(S)-2-((3-(6-amino-9H-purin-9-yl)propyl)amino)-3-phosphonopropanoic 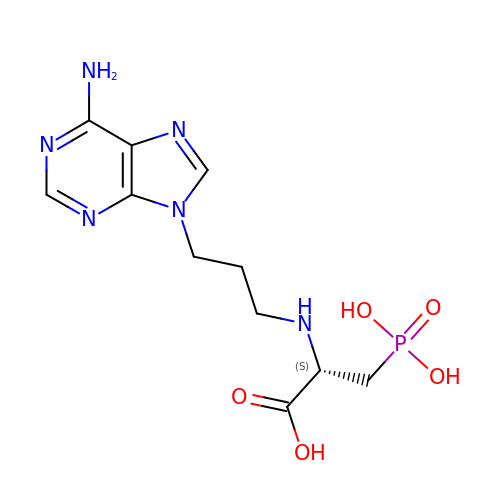acid | C11 H17 N6 O5 P | CFXXIYRDSBDIPF-SSDOTTSWSA-N Here we report that the 2-aminoisobutyric acid hydroxylase from Rhodococcus wratislaviensis, AibH1H2, requires manganese to functionalize a strong, aliphatic C–H bond (BDE = 100 kcal/mol). Structural and spectroscopic studies of this enzyme reveal a redox-active, heterobimetallic manganese–iron active site at the locus of O2 activation and substrate coordination. Metabolism of 2-aminoisobutyric acid (AIB) in Rhodococcus wratislaviensis proceeds via the initial, selective hydroxylation of the pro-(R) methyl group by the monooxygenase AibH1H2 to furnish α-methyl-d-serine (d-MeSer). Previously, recombinant expression of AibH1H2 in Escherichia coli enabled its structural characterization and revealed distinct mono- and dinuclear metal binding sites housed within the AibH1 and AibH2 protein subunits, respectively.

The expression of AibH1H2 in rich medium (lysogeny broth) furnished samples (LBAibH1H2) that contained ∼1.7 equiv of Fe and ∼1 equiv of Mn per AibH1H2 heterodimer (entry 2). The incorporation of tightly bound manganese ions was evident upon inspection of the electron paramagnetic resonance (EPR) spectra of exhaustively dialyzed samples. Unlike the case for FeAibH1H2, enzymatic assays employing LBAibH1H2 yielded substantial quantities of d-MeSer (33 equiv/AibH1H2). Since the protein structures of these two samples were found to be identical (RMSD = 0.34 Å over all atoms), our findings suggested an apparent requirement for one or more Mn ions in AibH1H2. For example, while our most active preparations have Mn in Site 0, other preparations, specifically LBAibH1H2, possess only 1 Mn ion and ∼2 Fe ions but are still competent for turnover. Although the precise location of the metals was not determined for this protein preparation, our biochemical data suggest that either (a) one of the Fe ions must occupy Site 0 or (b) there is a mixture of metalated and mismetalated protein if Mn must occupy Site 0 and Site 2. If the former is true, it would suggest that the metal identity of Site 0 is not specific and AibH1 may accept the most abundant metal available in the cellular environment.

>[4x]MGHHHHHHSGENLYFQSGGMVAPTSNPGVPDELDGVPAVVDCDVHAVLPSPHSLIPYLDEYWADQLVAQLAPTYEPNYHPRGSAIAQHSDASVDENGRAATTAENLVKDVFADGFTDFAVVNCLYGVQQIHQPRREMAHARALNHWIANEWLDKDDRLRASIVVPQGSPRAAAEEIDFWSGDKRFVQVLLLGQSELLYGREINWPIWEAAEAAGLPVTLHIGGVFRQAPTSVGWPASHLEWYVGQQSNIEAQLNSIISEGILQKFPKTKILLSELGFNWLPPFMWKFDKLWKSYRPDIPWVQESPLELIREHVRVTTSPSDGAEEAGRLDSIVDRLGSDRMLVYSSDYPHKHHSGPRDIENGTHSPELLDRIYRRNAFDLYNLVVPSPGKVG;>[4x]MTIIEHGSLGTLPAPSVTTGIVDADIHPVPQDGALEPYLDDRWKKHIREYGVRTTTGLQFISEYPQMYGGAMRADAWPESGYPGSDRELLRTQLLDKHNIQLGVLQCLAPGGQTLNPAGQALNQELAAALCRATNDWQLEHLVYPDPRMRAAIPVTFETPDYAVAEIERVGADPGVVAVLGTSKTLEPLGSRKYWPIYEASVAQNLPIQFHLSQGGGHANTGTGWTSYHTEYHTGHVQSFQSQLLSLVLSGTFDRFPTLKVMFVEGNVAHFAPLIQRMDYTWETLRGELPDLQRKPSEYIRDHIWASTQPIDEPEKPEHLAELLEEFCGDNVVFATDYPHFDFDDPETAFPRSFPVDLRDKILRGNGMRFFGVTNQAD> ASMQELYLLGVVPSRRFEAVVNSLSKTLDGPKTILEFWVVYRPKDVPPNLPRQPDSWLRLCSNIESHDETDTEWSKNTQWSMYLEGNSEPKREDKCGIRPVNRAKLTNGSVTEFVEKMGYEFSHEYIIQGLEYFFFDTTVRIYQTLIPSQQRSIKPPFHPMNEEQPWILHVYTHVADASNQVAMAKAEANLTKVKTLLSA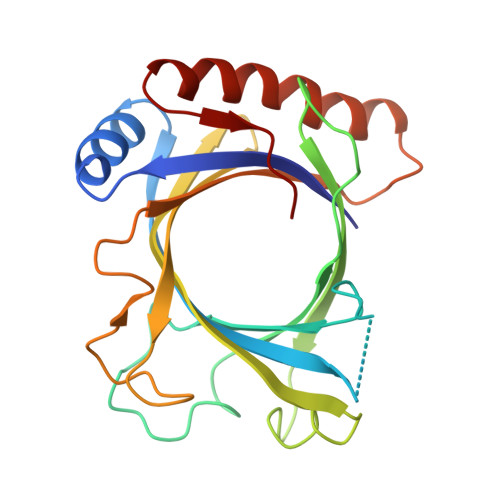FCDLKNVRL> AGGGGSSSGADHISLNPDLANEDEVNSCDYWRHCAVDGFLCSCCGGTTTTCPPGSTPSPISWIGTCHNPH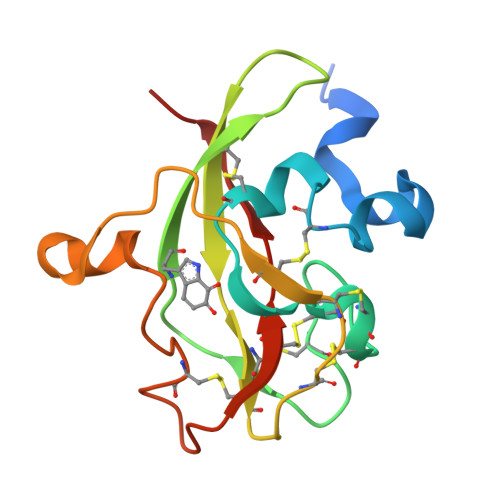DGKDYLISYHDCCGKTACGRCQCNTQTRERPGYEFFLHNDVNWCMANENSTFHCTTSVLVGLAKN>[2x]MAMPDVQYPINTYGWLKKAVALWADRDDDEFVNQIPNFINFAEKEIYRNLRIPPLEKEVYLDIKDGVAYIPPDYLEAQWMMRAKDGTIFQVTSPEEISYRRQHGTINPSHWNNQPVNFARFGSRFIFYPSIEADTPYYPDDGSPLIPAENSVILSYYADPPEFHEDTDTSTILTIAPELLLYFTLRHACLFVQDDNGVQKWSALGKAILDEMVEQNKKQEYSGSPIAIPNNMTRLQSSLPDIYGIRTSRV;>[3x]MAIETNAVVITDLNPLYPRDRDYIYEGAAQIRLIKQTLQNTFP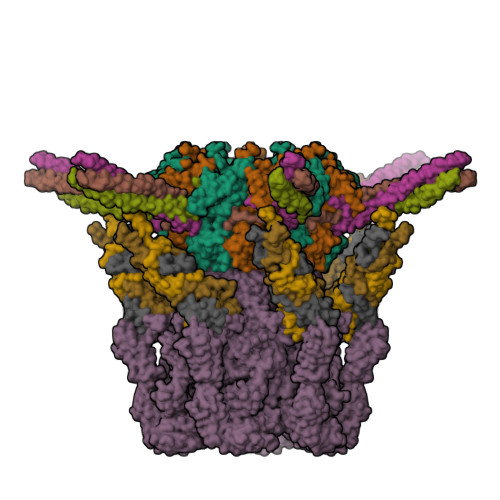NVTEPVDIDSDTFKIMSEKLKFTGDAMDVGGLMIKNVTPGTGDKDVVTKGQMEAFMKNWMENKLYRIGSYYITEEDINPGDSISLGFGSWAKVTGVIMGTGVVNPDGSVPNAQRVEFQAGGTGGRVFNTIRTENVPLMTVNGSSFSLSSNTHSHNMVFGRGDASGHNSSPNWYSPGGGYSQRTDNDTHTHTISGSVSLGRDDISRQPINTLPPFRAAHIWRRIS;>MIVYNNQAPDAVNNVGQFGATEGSIGAYKQAAEYAADSKYWALLAESKFGTIDDLIAEVERLYQQGVLMKQDIEDLKQDFKDQDARLMSLIAQTNAAVSDANNAVALINQKLIEVQNQLDVLLGMSVDVTTLPPGTPATGSFNPNTGVISLGIPEGEPGKDGSVKDLDTAPTGVPELGDLGFYVDKDDNTVHKTTLENIANLTPSVRSVSVNGGPALDGEVALTINKETVGLGNVLNVAQYSRQEINDKFDKTTKTYQSKAEAYADAQYRQVGEKVLVWEATKYEFYTVAANKTLTPVKTEGRILTVNSRSPDSSGNIDITIPTGNPSLYLGEMVMFPYDPSKNISYPGVLPADGRLVSKESASDLGPSLVSGQLPVVSETEWQSGAKQYFSWGKLADGITDADSTNFINIRLPDWTGGEAIRAPDSDKDSQYNGSVQAQKPYVVTVNNQAPDEITGNVNISRSILGAASSGANSDITSLSGLTTPLSISQGGTGAKDAASARSNLGLGSVSTLDNVPIASGGTGAGDAAGARFNLGLGNSATMNTGTNSDNVLKVGDFGIGRPDGALVFDTTSQDQLLAGLDTYGLCVFRNNQQIAAPWDIWNYSSNLFFRAGDTYSMISIPFESAGKIKVFGGASGSGWKTSRTVYDTVNTTVDVNGFIKAASPIVKVFHDGSFETNEQSDGVSVKKISTGVYLISGCLGLNSDAGWGGVDGGFEIPIDRNKQPRVWLDYEVKEDGSLLIKTYHRTHSTSPAFARNELEGFSDGDPVDIPKDAFISVRVEMPSK[3x];> MALYPIKSLGAVGVIADQAPTDLAPNAFTNAINARFVEQRVFKTGGNAPLSYVDEDKDLTPLSFVSMPFDYYSAGNSFLVVGTNKKLYKLTDESLTDISRKVATVTKKASASIKIYPVVSQIVPKESTISMNFNQTKNLEVSLLPADANNTNLIWEVSNSSYGSITVDPSDSKLATLTSFEKEGNLVVTISTANESVVAQIAVNIIDGDSGIFLSQDTVTIRKGGTTTLTAVTGKTPVTWSSNNASIVSVTPNANSLTAVITANGEGNVTITADNGTKTASCEIVSIPQIDSISLSQSDVTVSRGSQYILTATLSPANAPNQNITWTSSNPNIATVSGTSTQGTINALLAGFTEITATTEEGNRVAVCTVRVDLAGRTMRTSAMAFAAPVSESVETQEEEVVTPPESEETVYFAEPTSGIDTSGMYEGNNFYDYSNVNDIEGFARASLLATPLSSVTLDIVSASLDVGEEIVITATASPEGEYSYQWSVDKTGYVSTTSVTGKSIKLVALRKGEINVTCTVSQMTQKDYDAFDDYPWYHAVISNCAVATTHYETPQVKEFESEYFVDLPGWGEQTVVDNDGNPSVKKFNWKCERVRSFNNRLFALNMREANASGVTTNYPLRLRWSNFANENKAPTLWDDFAYDRVVSSDLASNIVGQTQALENGYAGYIDLADSNGSLIDILPLKDYLFVYTEFETYIGSPTNNTYQPLMFKKLFNDSGILAPECVVEVEGSHFVVTQNDVILHNGATKKSIASNRVKNMLINEVCLVNPLATRVHLHQDKKEVWVLYVGPGEPKESFACTKAAVWNYEFDTWSFRTIPYAQCIGLVDPPVLERGPIWSDFQEITWDDPSIKELVWRKDATNFRQRVTIVGSFLKGFYQVDVGALDYFYDRLNDVVIEKPLEMRLERTGIDFDNVTNEWNQKHINRFRPQTTGSGTYIFEAGGSQFSNEYGHPHTSKTYTIGVDRHVSVRLNHPYLFYNVIDNDVNSNAAINGLTIEFAVGGRR> MVFPMWTLKRQILILFNIILISKLLGARWFPKTLPCDVTLDVPKNHVIVDCTDKHLTEIPGGIPTNTTNLTLTINHIPDISPASFHRLDHLVEIDFRCNCVPIPLGSKNNMCIKRLQIKPRSFSGLTYLKSLYLDGNQLLEIPQGLPPSLQLLSLEANNIFSIRKENLTELANIEILYLGQNCYYRNPCYVSYSIEKDAFLNLTKLKVLSLKDNNVTAVPTVLPSTLTELYLYNNMIAKIQEDDFNNLNQLQILDLSGNCPRCYNAPFPCAPCKNNSPLQIPVNAFDALTELKVLRLHSNSLQHVPPRWFKNINKLQELDLSQNFLAKEIGDAKFLHFLPSLIQLDLSFNFELQVYRASMNLSQAFSSLKSLKILRIRGYVFKELKSFNLSPLHNLQNLEVLDLGTNFIKIANLSMFKQFKRLKVIDLSVNKISPSGDSSEVGFCSNARTSVESYEPQVLEQLHYFRYDKYARSCRFKNKEASFMSVNESCYKYGQTLDLSKNSIFFVKSSDFQHLSFLKCLNLSGNLISQTLNGSEFQPLAELRYLDFSNNRLDLLHSTAFEELHKLEVLDISSNSHYFQSEGITHMLNFTKNLKVLQKLMMNDNDISSSTSRTMESESLRTLEFRGNHLDVLWREGDNRYLQLFKNLLKLEELDISKNSLSFLPSGVFDGMPPNLKNLSLAKNGLKSFSWKKLQCLKNLETLDLSHNQLTTVPERLSNCSRSLKNLILKNNQIRSLTKYFLQDA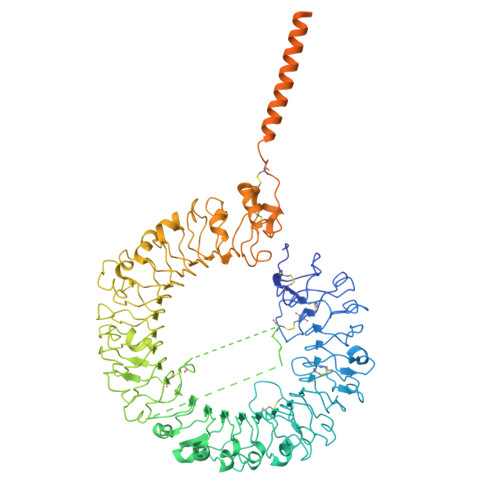FQLRYLDLSSNKIQMIQKTSFPENVLNNLKMLLLHHNRFLCTCDAVWFVWWVNHTEVTIPYLATDVTCVGPGAHKGQSVISLDLYTCELDLTNLILFSLSISVSLFLMVMMTASHLYFWDVWYIYHFCKAKIKGYQRLISPDCCYDAFIVYDTKDPAVTEWVLAELVAKLEDPREKHFNLCLEERDWLPGQPVLENLSQSIQLSKKTVFVMTDKYAKTENFKIAFYLSHQRLMDEKVDVIILIFLEKPFQKSKFLQLRKRLCGSSVLEWPTNPQAHPYFWQCLKNALATDNHVAYSQVFKETV Farnesyl pyrophosphate synthase (FPPS; EC 2.5.1.10) is a promising antibiotic drug target as it represents the point of convergence of these two pathways. The enzyme belongs to a large group of prenyltransferases responsible for the principal bond-forming reactions of isoprenoid biosynthesis. The mevalonate and nonmevalonate pathways both produce isopentenyl pyrophosphate (IPP), which along with its isomer dimethyl­allyl diphosphate (DMAPP) is converted through a ‘head-to-tail’ condensation reaction to form geranyl diphosphate (GPP) by FPPS. In summary, this work provides the first functional and structural insights into FPPS from the opportunistic pathogen P. aeruginosa.

In order to investigate the structural basis of inhibition of PaFPPS by N-BPs, we determined the structure of the enzyme in complex with ibandronate (Bonviva) to 1.85 Å resolution. We note that also in the ibandronate complex the active site is in the open conformation and the lid region is disordered. Three ibandronate molecules were bound in the active site in this subunit. Molecule BFQ1299 is located in site S1, the common binding site for the DMAPP/GPP substrates and N-BP inhibitors in other FPPSs. The hydrophobic tail of this ibandronate molecule extends into the same pocket as the isoprenyl tail of GPP, which is lined by residues Tyr78, Ser79, Leu111, Met153, Val154, Gln157 and Lys180. Like the diphosphate group of GPP (see above), the bisphosphonate group is anchored to the protein via two Mg2+ ions (denoted Mg1294 and Mg1295 in this complex), which in turn are bound to the enzyme by two aspartate residues from motif I: Asp81 and Asp83. A third Mg2+ ion (Mg1300) is bound at the opposite site of the bisphosphonate group and completes the trinuclear metal site seen in FPPS–ligand complexes from other species. However, owing to the absence of the hinge motion, motif II is not close enough to provide ligands to this metal ion. In place of these stabilizing interactions from motif II, Mg1300 together with two additional Mg2+ ions (Mg1301 and Mg1302) provides the anchoring point of two additional ibandronate molecules that are bound at the active site. However, we consider the binding of these additional inhibitor molecules to be a consequence of the open conformation of the enzyme in the crystal lattice rather than a novel, alternative mode of inhibition by N-BPs in PaFPPS.

>SMIAAYQARCQARVDAALDALFVAPREELQRLYEAMRYSVMNGGKRVRPLLAYAACEALGGAPQRADAAACAVELIHAYSLVHDDLPAMDDDDLRRGQPTTHRAFDEATAILAADGLQALAFEVLADTRRNPQEHAVCLEMLTRLARAAGSAGMVGGQAIDLGSVGVALDQAALEVMHRHKTGALIEASVRLGALASGRAEPASLAALERYAEAIGLAFQVQDDILDVESDTATLGKTQGKDQAHNKPTYPALLGLEAAKGYALELRDLALAALDGFPPSADPLRQLARYIVERRN[2x]> MFDFRLLLLCLGAFLTFTNASPSPYPQSSNAPAALNACLASKKVPYIPRDSAQWVKEVKPYNLRLAYTPAAIALPTTVKHISDAVKCGDQNKVRVSAKSGGHSYGSFGYGGENGHLVIVVDAMDTVTLNKDMSCTVQAGARLGHVATDLFQFGKRAIPHGSCPGVGIAGHALHGGYGFASRTHGLTLDTFLGATIVLTNGTIRYAADWEYYDLTWALRGAGSSFGIVAELGFQTFAAPETVTPFSIELDWNENEAVEGLLAMQKFAVTAPKELNMQIYMGPSGQTIQGVYYGTRANLNTALRPLLGDLGAQISTASTGGWIQMLNKYANGQALDQRRPYDQHSTFYSTSLMTKALTRNQVKSFARTLFDNMNDSDARHTWYILIDLFGGPNSAVTNAKTLFTDLPINSAFPHRDKLLLWQFSDHGNYATHANNGFTVLKRFRDSVTKTMADGDWGMYANYLDTQLSNEEAVKRYYGKS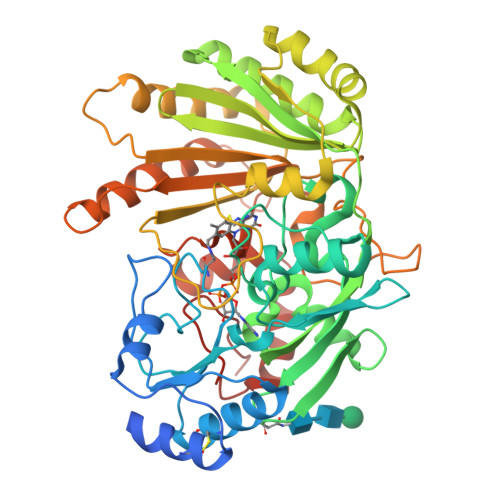LPKLKKLKAELDPKDMFWNPQGIRPAAAHHHHHH>GPGSMVSEKGRLFTSESVTEGHPDKICDAISDSVLDALLAADPRSRVAVETLVTTGQVHVVGEVTTSAKEAFA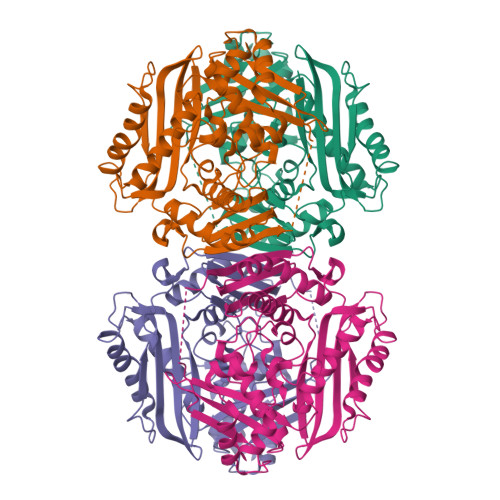DITNTVRARILEIGYDSSDKGFDGATCGVNIGIGAQSPDIAQGVDTAHEARVEGAADPLDSQGAGDQGLMFGYAINATPELMPLPIALAHRLSRRLTEVRKNGVLPYLRPDGKTQVTIAYEDNVPVRLDTVVISTQHAADIDLEKTLDPDIREKVLNTVLDDLAHETLDASTVRVLVNPTGKFVLGGPMGDAGLTGRKIIVDTYGGWARHGGGAFSGKDPSKVDRSAAYAMRWVAKNVVAAGLAERVEVQVAYAIGKAAPVGLFVETFGTETEDPVKIEKAIGEVFDLRPGAIIRDLNLLRPIYAPTAAYGHFGRTDVELPWEQLDKVDDLKRAI[4x]> ANLNGTLMQYFEWYMPNDGQHWKRLQNDSAYLAEHGITAVWIPPAYKGTSQADVGYGAYDLYDLGEFHQKGTVRTKYGTKGELQSAIKSLHSRDINVYGDVVINHKGGADATEDVTAVEVDPADRNRVISGEHLIK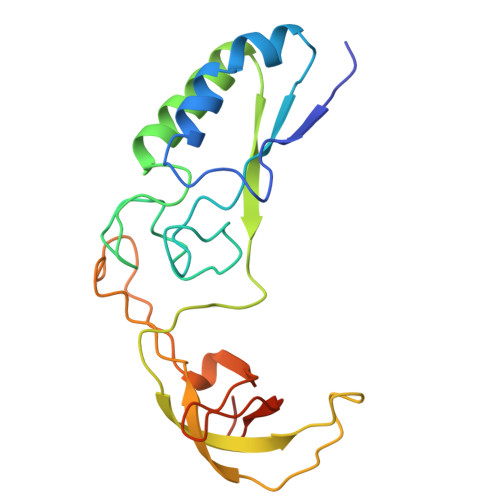AWTHFHFPGRGSTYSDFKWHWYHFDGTDWDESRKLNRIYKFQGKAWDWEVSNE>GAMGPTSNDACLSIVHSLMCHRQGGESETFAKRAIESLVKKLKEKKDELDSLITAITTNGAHPSKCVTIQRTLDGRLQVAGRKGFPHVIYARLWRWPDLHKNELKHVKYCQYAFDLKCDSVCVNPYHYERVVSPG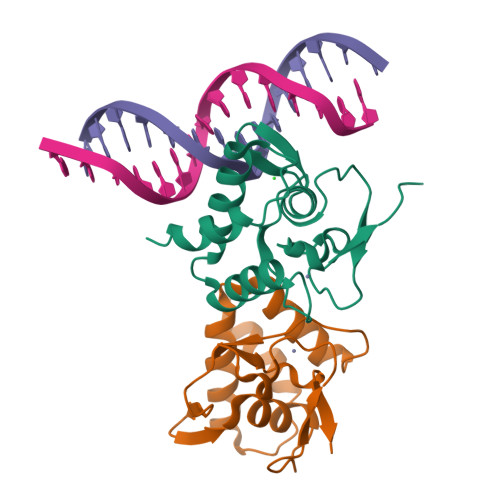[2x]> SSEQLKHCNGILKELLSKKHAAYAWPFYKPVDASALGLHDYHDIIKHPMDLSTVKRKMENRDYRD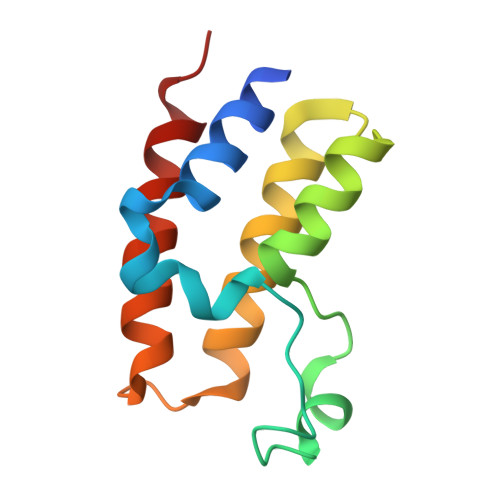AQEFAADVRLMFSNCYKYNPPDHDVVAMARKLQDVFEFRYAKMP6-[(3,5-dichloropyridin-4-yl)methoxy]-1-{[3-(trifluoromethyl)phenyl]sulfonyl}-2,3-dihydro-1H-indole 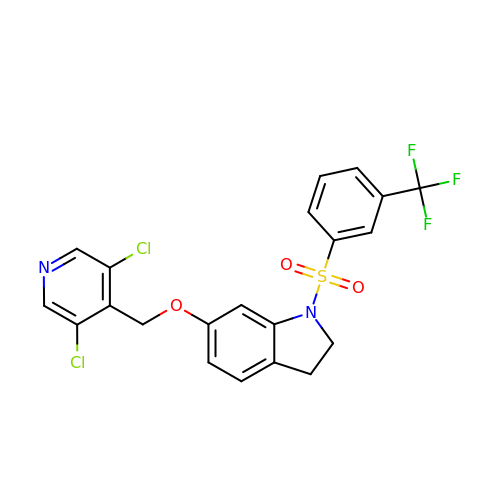| C21 H15 Cl2 F3 N2 O3 S | PXLLMOZEQWSZPR-UHFFFAOYSA-N> MIKTRIEEVQLQFLTGNTELTHLKVSNDQLIVTTQRTIYRINLQDPAIVNHFDCPLSKELETIMNVHVSPMGSVILIRTNFGRYMLLKDGEFTQLNKIKNLDLSSLHWINETTFLMGIKKTPKLYRVELTGKDITTKLWYE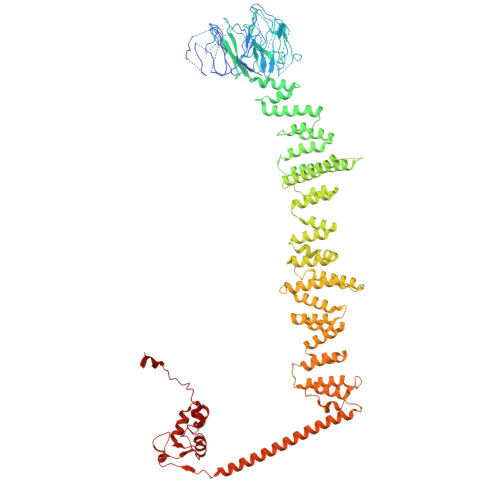NKKLSGGIDGIAYWEGSLLLTIKDNILYWRDVTNMKFPLVLPDESEQFERLKHHAIKKFDSYNGLFAWVTSNGIVFGDLKEKQMEKDPASNNFGKFLSSSKVLLNFELPDYQNDKDHLIKDIVLTAFHILLLRKNTVTMVSQLNNDVVFHETIPRHQLTGSNTDSNEKFLGLVRDSVKETFWCFSNINVFEIIIENEPNSVWNLLVRDNKFDKALSLKGLTVREIESVKLSKAMYLFHTAKDFHSAAQTLGSMKDLSHFGEIALNFLQIKDYNDLNVILIKQLDNVPWKSTQVVLSSWIIWNFMKQLNDIELKINTTKPASTDEDNLLNWNLNLKEKSNELTKFLESHLEKLDNETVYQIMSKQNRQNELLIFASLINDMKFLLSFWIDQGNWYESLKILLTINNHDLVYKYSLILLLNSPEATVSTWMKIKDLDPNKLIPTILKFFTNWQNNSKLITNISEYPENYSLTYLKWCVREVPKMCNPIVYNSILYMMITDPRNDMILENDIIKFMKSNENKYDLNFQLRLSLKFKKTKTSIFLLTRLNLFEDAIDLALKNNLIDDCKVIVNDEILIEDYKLRKRLWLKIAKHLLLSMKDIDIKQLIRTILNDSNEILTIKDLLPFFNEYTTIANLKEELIKFLENHNMKMNEISEDIINSKNLKVEINTEISKFNEIYRILEPGKSCDECGKFLQIKKFIVFPCGHCFHWNCIIRVILNSNDYNLRQKTENFLKAKSKHNLNDLENIIVEKCGLCSDININKIDQPISIDETELAKWNE> GFNYDEAQVPKYTLPDPLVMVDGTKVTSAKQWNDKRRDEVQQLFEAYMYGKVPDGETELIFTDAKGERALGGAAIRKQVKISFGEKEDAPAMDLLIYLPADAKVRVPVFLGLNFHGNHTIHKDKEIWLTESWVRTNKKFGITKNKANELSRGVAAGRWQIEKAIAKGYGVATIYCGDIDPDFNFPSNGIQAYYYKK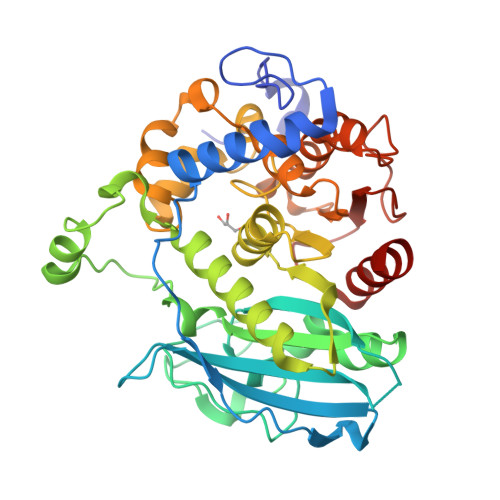DQTIPEKGQWGTIAAWAFGLSCAMDYFETDTDIDHKKVAVLGHSRLGKTSLWAGAIDTRFALTISNCSGCGGAALSRRRFGETVRRINTSFPHWFCSRFHQYNDKEDKLPIDQHMLIALCAPRPVLINSATEDKWADPHGEFLAAQGADAVYRMLGTGGLDAKKWPEPNKLVKSTIGYHLRPGKHDVTARDWDVYIEFADHHM>[2x]ATTLYENKTGTEDGYDYELWKDSGNTSMILNGGGTFSCQWSNINNCLFRKGKKFGGNQSYQQIGNISFDYGCDYHPNGNSYLCVYGWTTSPLVEFYIVDSWGSWRPPGG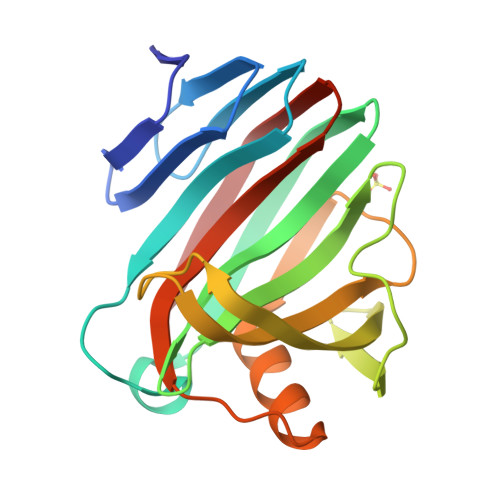SPKGQIYVDGGTYDVYETTRVNQPSIQGNTTFQQYFSVRTERRTSGTINVTEHFKAWERMGMRMGNIYEAALNVEGYQSSGSANVYKNNMTIG> GPDSMDPYDALGNAVDFLDA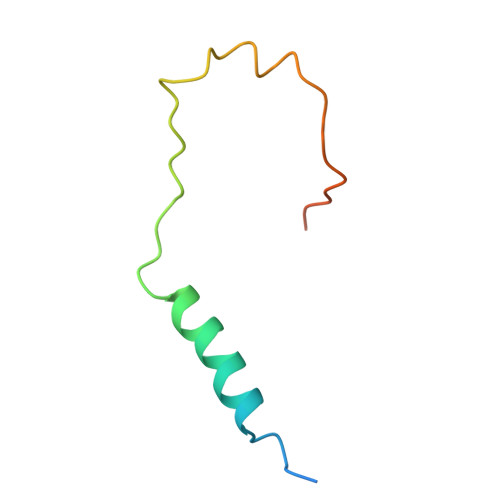RLHSLSNYQKRPISIKSNIIDEETYKKYPSLFSWDKIEASKKSDN> GSSDDRPLLERVKDVVADQLGVDR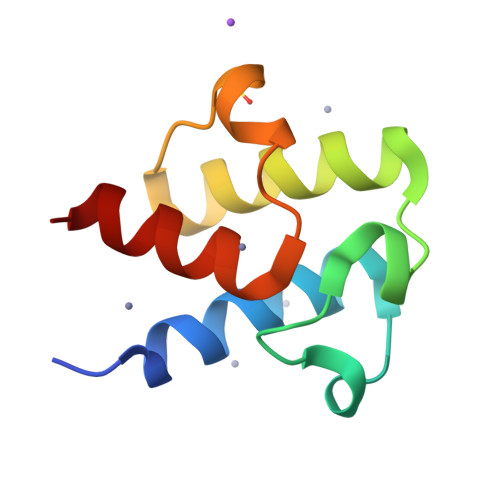ARINPESNFIKDLDADSLDSVELVMAFEEKFGVSIPDEEASKIATVQDALSYIEKAKS>SYLGSEFDNVELKDLANVLSFGEAKLGDNGQKFNFLFHTASSNVWVPSIKCTSESCESKNHYDSSKSKTYEKDDTPVKLTSKAGTISGIFSKDLVTIGKLSVPYKFIEMTEIVGFEPFYSESDVDGVFGLGWKDLSIGSIDPYIVELKTQNKIEQAVYSIYLPPENKNKGYLTIGGIEERFFDGPLNYEKLNHDLMWQVD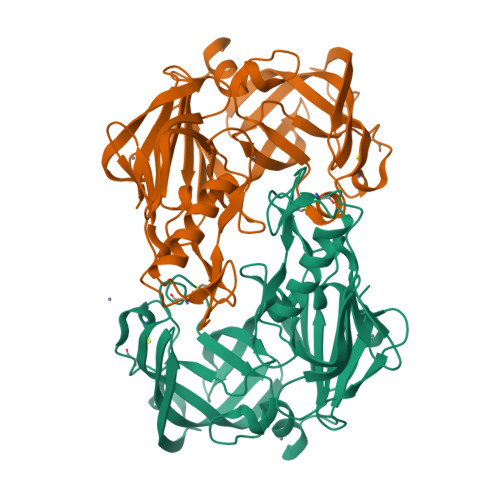LDVHFGNVSSKKANVILDSATSVITVPTEFFNQFVESASVFKVPFLSLYVTTCGNTKLPTLEYRSPNKVYTLEPKQYLEPLENIFSALCMLNIVPIDLEKNTFVLGDPFMRKYFTVYDYDNHTVGFALAKNL[2x]>MRGSHHHHHHGSASAWPEEKNYHQPAILNSSALRQIAEGTSISEMWQNDLQPLLIERYPGSPGSYAARQHIMQRIQRLQADWVLEIDTFLSQTPEGERSFSNIISTLNPTAKRHLVLACHYDSKYFSHWNNRVFVGATDSAVPCAMMLELARALDKKLLSLKTVSDSKPDLSLQLIFFDGEEAFLHWSPQDSLYGSRHLAAKMASTPHPPGARGTSQLHGMDLLVLLDLIGAPNPTFPNFFPNSARWFERLQAIEHELHELGLLKDHSLEGRYFQNYSYGGVIQDDHIPFLRRGVPVLHLIPSPFPEVWHTMDDNEENLDEST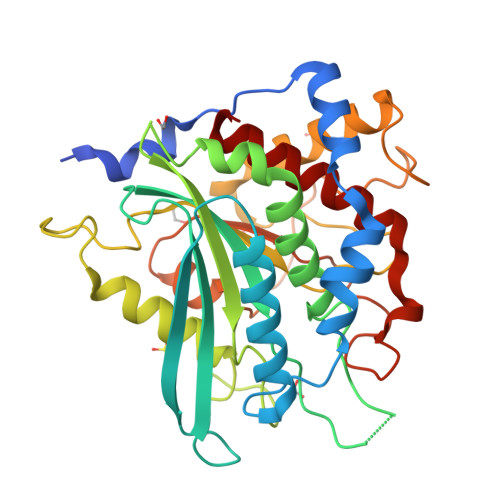IDNLNKILQVFVLEYLHL[3x]>MGDNEKINREALAPREYGESLELGIEFTTTEEIEV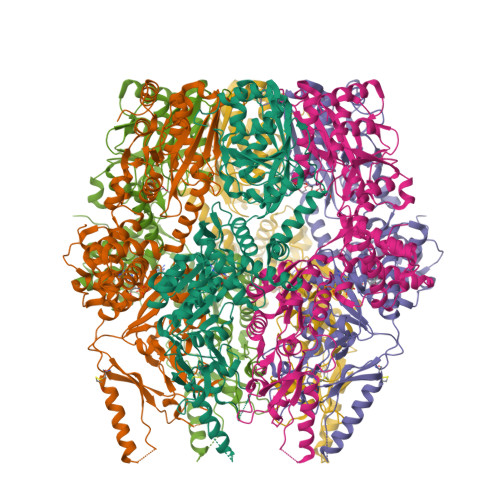PEKLIDQVIGQEHAVEVIKTAANQKRHVLLIGEPGTGKSMLGQAMAELLPTETLEDILVFPNPEDENMPRIKTVPACQGRRIVEKYREKAKSQESVKSSNMRLKSTVLVPKLLVDNCGRTKAPFIDATGAHAGALLGDVRHDPFQSGGLGTPAHERVEPGMIHRAHKGVLFIDEIATLSLKMQQSLLTAMQEKKFPITGQSEMSSGAMVRTEPVPCDFVLVAAGNLDTVDKMHPALRSRIRGYGYEVYMRTTMPDTIENRRKLVQFVAQEVKRDGKIPHFTKEAVEEIVREAQKRAGRKGHLTLRLRDLGGIVRAAGDIAVKKGKKYVEREDVIEAVKMAKPLEKQLADWYIERKKEYQVIKTEGSEIGRVNGLAVIGEQSGIVLPIEAVVAPAASKEEGKIIVTGKLGEIAKEAVQNVSAIIKRYKGEDISRYDIHVQFLQTYEGVEGDAASISVATAVISALEGIPIRQDVAMTGSLSVRGEVLPIGGATPAIEAAIEAGIKMVIIPKSNEKDVFLSKDKAEKIQIFPVETIDEVLEIALEESEKKRELLRRIRETLPLSLHHHHHH[2x]>MEAVPRMPMIWLD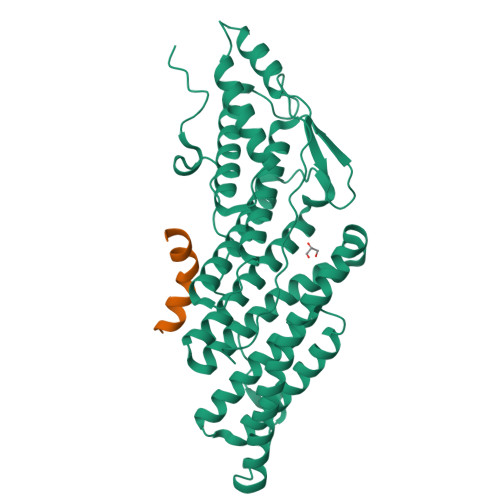LKEAGDFHFQPAVKKFVLKAAGENPEAYNEELKKLELLRQNAVRVPRDFEGCSVLRKYLGQLHYLQSRVPMGSGQEAAVPVTWTEIFSGKSVAHEDIKYEQACILYNLGALHSMLGAMDKRVSEEGMKVSCTHFQCAAGAFAYLREHFPQAYSVDMSRQILTLNVNLMLGQAQECLLEKSMLDNRKSFLVARISAQVVDYYKEACRALENPDTASLLGRIQKDWKKLVQMKIYYFAAVAHLHMGKQAEEQQKFGERVAYFQSALDKLNEAIKLAKGQPDTVQDALRFTMDVIGGKYNSAKKDNDFIYHEAVPALDTLQPVKGAPLVKPLPVNPTDPAVTGPDIFAKLV[2x];>LNVKVLEALELYNKLVNEAPV[2x]>SNKKTKLIHGGHTTDDYTGAVTTPIYQTSTYLQDDIGDLRQGYEYSRTANPTRSSVESVIATLENGKHGFAFSSGVAAISAVVMLLDKGDHIILNSDVYGGTYRALTKVFTRFGIEVDFVDTTHTDSIVQAIRPTTKMLFIETPSNPLLRVTDIKKSAEIAKEHGLISVVDNTFMTPYYQNPLDLGIDIVLHSATKYLGGHSDVVAGLVATSDDKLAERLAFISNSTGGILGPQDSYLLVRGIKTLGLRMEQINRSVIEIIKMLQAHPAVQQVFHPSIESHLNHDVHMAQADGHTGVIAFEVKNTESAKQLIKATSYYTLAESLGAVESLISVPA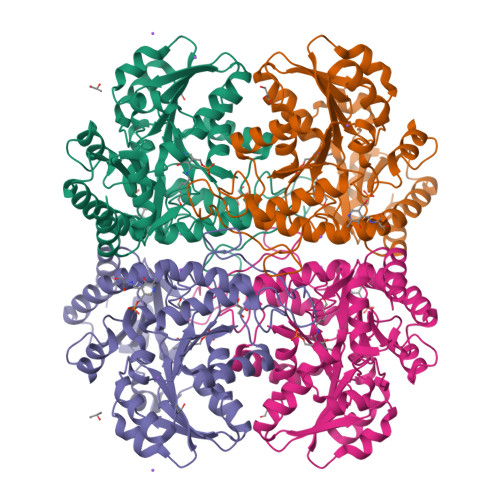LMTHASIPADIRAKEGITDGLVRISVGIEDTEDLVDDLKQALDTL[2x]>[2x]SKALLKGVRDFNPISACVCLLENSSDGHSERLFGIGFGPYIIANQHLFRRNNGELT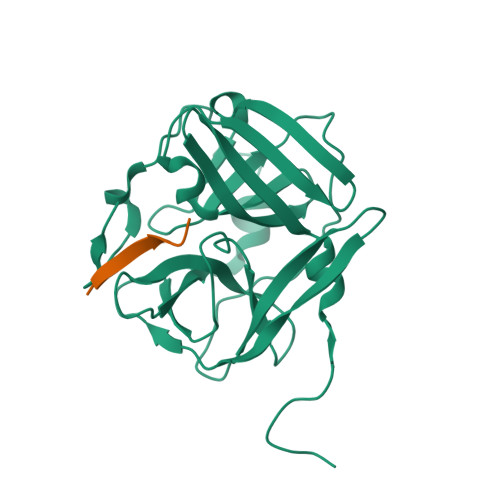IKTMHGEFAVANSTQLQMKPVEGRDIIVIKMAKDFPPFPQKLKFRQPTIKDRVCMVSTNFQQKSVSSLVSESSHIVHKEDTSFWQHWITTKDGQAGSPLVSIIDGNILGIHSLTHTTNGSNYFVEFPEKFVATYLDAADGWCKNWKFNADKISWGSFTLVEDAPEDDFMAKKTVAAIMDDLVRTQ;>[2x]ETVRFQSD> MAHHHHHHGGSEPFYITTAIAYPNGVPHIGHAYEYIATDAIARFKRLDGYDVRYLTGTDVHGQKMAETAAKEGIPAAELARRNSDVFQRLQEKLNISFDRFIRTSDADHYEASKAIWKRMADAGDIYLDAYKGWYSIRDERFFTENETTEQPDGTRIATETGAPVTWTEEQTYFFRLSAYTDRLLALYEEHPEFIGPDARRNEIVSFVSGGLKDLSISRTTFDWGVPVPDHPDHVMYVWVDALTNYLTGVGFPDTESESFRRYWPADLHMIGKDIIRFHTVYWPAFLMSAGLPLPKRIFAHGWLLNRGEKMSKSIGNVVDPVNLVDTFGLDQVRYFLLREVPFGQDGSYNEDAIIGRVNADLANELGNLAQRSLSMVAKNLGAAVPDPGEFTDEDTALLAAADALLERVREHFDVPAMHLAL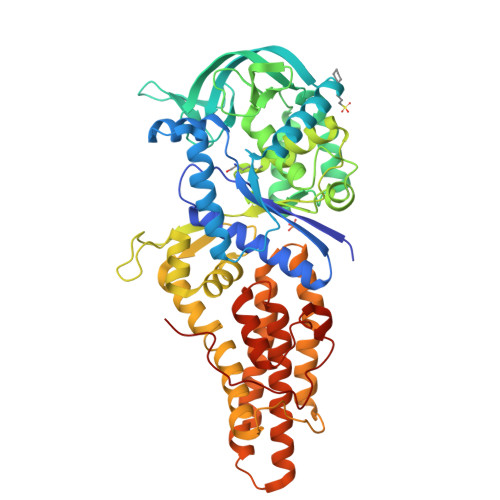EAIWSVLGAANRYFSAQEPWVLRKSDAAEDQQRFRTVLYTTLEVVRIASLLLQPVMPESTAKLLDLLGQPTDERDFSAIANRIKPGTSLPAPSGIFPRYQND> NVNQTMADNQ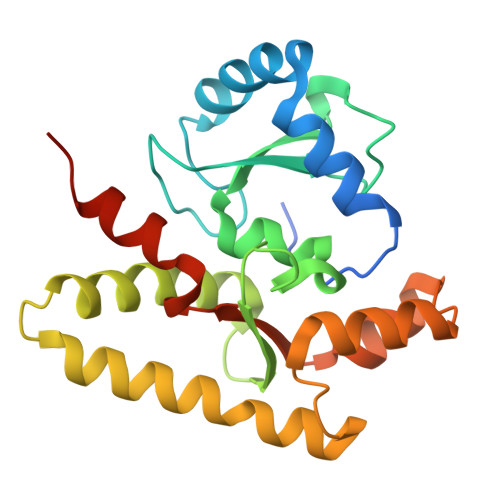QRCELKLIASPGSWRLYSARKIDERFKSYEQKIFQRDRYTCQFCGFQARLYQDIVNLDGDYTNNRLSNLVTACCFCAQCFFVESVGVGGYGGGTLIYLPELTQAELNSLCHVLFCAITNDTGYKSSAQNIYRSFKFRSQIVEEKFGEGTSDPAIFGQLMIDSGVNSEEIREKLFKNIRLLPSRAKFRKQIEKWAASALEEIAD> RKTITGVFNSFDSLTWTRSVEYVYKGPETPTWNAVLGWSLNSTTADPGDTFTLILPCVFKFITTQTSVDLTADGVSYATCDFNAGEEFTTFSSLSCTVNSVSVSYARVSGTVKLPITFNVGGTGSSVDLADSKCFTAGKNTVTFMDGDTKISTTVDFDASPVSPSGYITSSRIIPSLNKLSSLFVVPQCENGYTSGIMG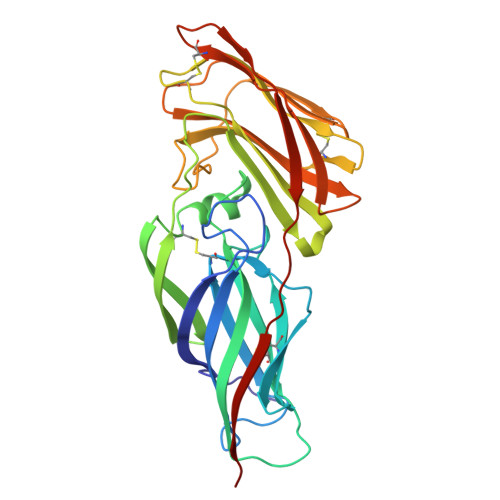FVASNGATIDCSNVNIGISKGLNDWNFPVSSESFSYTKTCTSTSITVEFQNVPAGYRPFVDAYISAENIDKYTLTYANEYTCENGNTVVDPFTLTWWGYKNSEADSDGDVIVV> MGSSHHHHHHSQDPKISDVVVELFREAAIYLPEDVKNALEEAYKKESSEISKNTLKAIIENNKIAEETQVPLCQDTGVPIVFLKI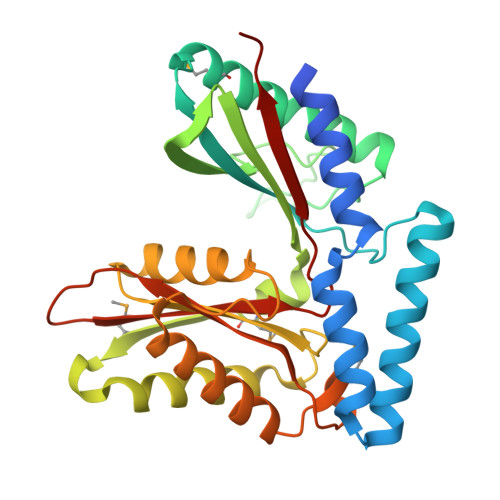GKNINSSEIMKIIEEIKEGVKKATEEVPLRPNVVHPLTRENFKTNVGLNSPFINIEFDESLDREIEIIAFPKGAGSENMSALKMLKPSDGIEGIKNFVLETIANAGGKPCPPIVVGIGIGGTADVALKLAKKALLRKIGERHRDKEIANLEKELLEKINSLGIGAMGLGGDITALDVFIEIAGCHTASLPVGICIQCWADRRAIKRIKLDAKL The glycosyltransferase Kcn28, which is unique among all CCNP BGCs, was expected to transfer a glycosyl group onto either the terminal COOH (5 and 6) or OH group (9 and 10). The monomeric Kcn28 contains two Rossmann-like β/α/β domains. The N-terminal domain from residues 6–208 is a substrate binding domain consisting of seven parallel β-strands that are flanked by seven α-helices, while the C-terminal domain comprising residues 229–392 is a UDP-sugar binding domain with six parallel β-strands surrounded by seven α-helices. A glycosyltransferase with relatively broad substrate specificity transfers sugars to the newly generated OH/COOH group.

We further attempted to understand the structural basis of the Kcn28-catalyzed enzymatic reaction. Crystal structures of Kcn28 as a free enzyme and in a binary complex (with 9) were obtained at 2.50 and 2.24 Å resolution, respectively (Fig. 4A and B and Table S17†). Superposition of free and complexed structures revealed a global conformational change.

>[4x]GSHMPRPGHIAMVSVPSRGHLHPSLELIRELVARGHRVTYANDPSVAAAVTETGAELVPYTSALPSTDTTEGRVTDQIAQMDVFLDDAVGMLPQLRAAYEEDRPDVFLYDVLAYPARVLAMNWGIPSIQISPTWVMPEKYRERMAPVVEQLKQDPRGAAHYRRFDAWLEDSGVPGIDAGDLVNLPERSLVLVPRFLQPDADDVDEKRFTFIGPCLGRRAHQGDWKRPAGAEKVALVSLGSHLTNQLPFYETCVEVFAALPDWHLVLQIGRHVDAGELGELPPNVEVHNWVPQLAVLEQADVFVTHGGMGGIQEGLFSGVPMVVAPQANDQPANAESVVGLGIARRIDIATVTPDRLRAAVVELASDPAVAERLSGLRRELRAHGGTMRAADLIERQLPA methyl 4,9-di-O-acetyl-5-acetamido-3,5-dideoxy-D-glycero-alpha-D-galacto-non-2-ulopyranosidonic 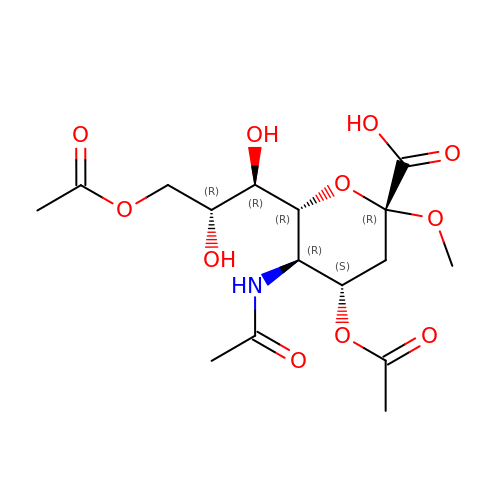acid | C16 H25 N O11 | PJCATKAGSUTUJA-NVWMEEMDSA-N> MSSVTWAPGNYPSTRRSDHVDTYQSASKGEVPVPDPYQWLEESTDEVDKWTTAQADLAQSYLDQNADIQKLAEKFRASRNYAKFSAPTLLDDGHWYWFYNRGLQSQSVLYRSKEPALPDFSKGDDNVGDVFFDPNVLAADGSAGMVLCKFSPDGKFFAYAVSHLGGDYSTIYVRSTSSPLSQASVAQGVDGRLSDEVKWFKFSTIIWTKDSKGFLYQRYPARERHEGTRSDRNAMMCYHKVGTTQEEDIIVYQDNEHPEWIYGADTSEDGKYLYLYQFKDTSKKNLLWVAELDEDGVKSGIHWRKVVNEYAADYNIITNHGSLVYIKTNLNAPQYKVITIDLSKDEPEIRDFIPEEKDAKLAQVNCANEEYFVAIYKRNVKDEIYLYSKAGVQLTRLAPDFVGAASIANRQKQTHFFLTLSGFNTPGTIARYDFTAPETQRFSILRTTKVNELDPDDFESTQVWYESKDGTKIPMFIVRHKSTKFDGTAAAIQYGYGGFATSADPFFSPIILTFLQTYGAIFAVPSIRGGGEFGEEWHKGGRRETKVNTFDDFIAAAQFLVKNKYAAPGKVAINGASNGGLLVMGSIVRAPEGTFGAAVPEGGVADLLKFHKFTGGQAWISEYGNPSIPEEFDYIYPLSPVHNVRTDKVMPATLITVNIGDGRVVPMHSFKFIATLQHNVPQNPHPLLIKIDKSWLGHGMGKPTDKNVKDAADKWGFIARALGLELKTVE

GmPOPB is the macrocyclase responsible for macrocyclization of amatoxins, eight amino-acid ribosomal peptides with the core sequence IWGIGC(N/D)P. Amatoxins are cyclic peptides further modified by a characteristic sulfoxide cross-link between tryptophan and a cysteine, and hydroxylation (the extent of which vary). GmPOPB is an unusual enzyme catalyzing, depending on substrate length, proteolysis, or macrocyclization using the same catalytic machinery. The protein contains two domains as observed in other POP enzymes. The domain containing the putative catalytic residues (Ser577, Asp661, His698) comprises residues 1–81 and 450–728, and the other domain is a seven bladed β-propeller, comprising residues 82–449.

The apo protein crystals belong to space group P212121, with one monomer in the asymmetric unit. In the apo structure, the two domains are in an “open” conformation, in an arrangement reminiscent of a hinged lid on a bottle. This open conformation has been observed in other POPs in crystal form when free of ligand. The catalytic serine sits at the tip of a loop and points toward the β-propeller domain. The side chain oxygen of Ser577 is 5.6 Å from the side chain carboxylate of Asp661; His698 is on a loop that is disordered. Ser577 and Asp661 of GmPOPB occupy the same position as Ser554 and Asp641 in the porcine proline oligopeptidase structure. Comparison to the apo structure reveals that binding of substrate induces no significant changes in the core of the propeller domain (rmsd of 0.75 Å over 360 Cα positions for the S577A structures). The changes that occur (relative to the apo structure) are in loops around the catalytic site.> SMKTKLMTLQDATGFFRDGMTIMVGGFMGIGTPSRLVEALLESGVRDLTLIANDTAFVDTGIGPLI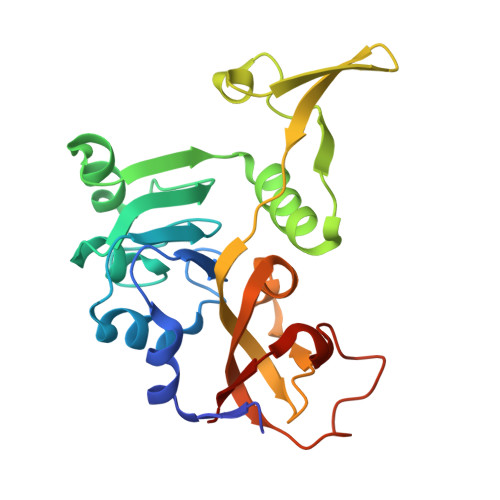VNGRVRKVIASHIGTNPETGRRMISGEMDVVLVPQGTLIEQIRCGGAGLGGFLTPTGVGTVVEEGKQTLTLDGKTWLLERPLRADLALIRAHRCDTLGNLTYQLSARNFNPLIALAADITLVEPDELVETGELQPDHIVTPGAVIDHIIVSQESK>MAANPFSDVTPDSWAYQAVSQLAQAGIVNGYPDGTFKGQNNITRYEMAQMVAKAMANQDRANAEQQAMINRLADEFSNELNNLGVRV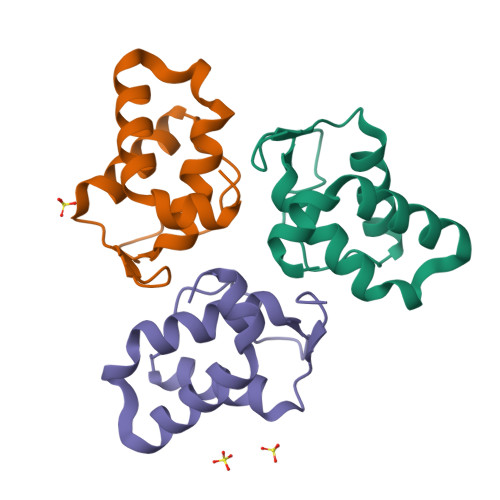SLEHHHHHH[3x]Here we report cryo-EM structures of the HEAT-repeat protein Met18 from Saccharomyces cerevisiae, a key component of the CIA targeting complex (CTC) that identifies cytosolic and nuclear client proteins and delivers a mature iron-sulfur cluster. Met18 is a 118 kDa alpha solenoid protein comprised entirely of HEAT (Huntingtin, elongation factor 3 (EF3) repeats, protein phosphatase 1A, and the yeast kinase TOR1) repeats. ScMet18 has a curved S-shaped structure comprised of 23 HEAT-repeat (HR) units; each HR contains two α-helices that are connected by loops. We find that in the absence of other CTC proteins, Met18 adopts tetrameric and hexameric states.

To the best of our knowledge, our cryo-EM structure shows for the first time that ScMet18 can form an intertwined hexamer in the absence of other proteins. Our final model contains six copies of Met18 with each protomer consisting of residues 9-1029 with two loops missing at residues 225–241 and 315–337. The hexamer is 154 Å long and has both 3-fold and 2-fold symmetry. For all chains, the N-terminus is solvent-exposed, and the C-terminus is buried. Each chain of the hexamer interacts with 4 other chains (i.e., chain A touches chains B, C, D, and F, but not chain E). The hexamer is comprised of trimers and dimers where chains A, B, and C and chains D, E, and F can form trimers, and chains A and F, B and E, and C and D form dimers. Notably, the dimer from ScMet18 hexamer is not the same as the dimer observed in the crystal structure of MmMet18 in complex with DmCia2b-DmCia1. The curvature of ScMet18 differs from what has been observed previously with the MmMet18 protein in complex with DmCia2-DmCia1; there is a 44 Å shift in the N-terminus of ScMet18 compared to MmMet18. Notably, residues that appeared to be involved in binding Cia2 (R1010, R1013, R1020) are buried in both the hexameric and tetrameric states of ScMet18, indicating that ScCia2 cannot bind to ScMet18 without disrupting these higher order oligomeric states.

>MTPDELNSAVVTFMANLNIDDSKANETASTVTDSIVHRSIKLLEVVVALKDYFLSENEVERKKALTCLTTILAKTPKDHLSKNECSVIFQFYQSKLDDQALAKEVLEGFAALAPMKYVSINEIAQLLRLLLDNYQQGQHLASTRLWPFKILRKIFDRFFVNGSSTEQVKRINDLFIETFLHVANGEKDPRNLLLSFALNKSITSSLQNVENFKEDLFDVLFCYFPITFKPPKHDPYKISNQDLKTALRSAITATPLFAEDAYSNLLDKLTASSPVVKNDTLLTLLECVRKFGGSSILENWTLLWNALKFEIMQNSEGNENTLLNPYNKDQQSDDVGQYTNYDACLKIINLMALQLYNFDKVSFEKFFTHVLDELKPNFKYEKDLKQTCQILSAIGSGNVEIFNKVISSTFPLFLINTSEVAKLKLLIMNFSFFVDSYIDLFGRTSKESLGTPVPNNKMAEYKDEIIMILSMALTRSSKAEVTIRTLSVIQFTKMIKMKGFLTPEEVSLIIQYFTEEILTDNNKNIYYACLEGLKTISEIYEDLVFEISLKKLLDLLPDCFEEKIRVNDEENIHIETILKIILDFTTSRHILVKESITFLATKLNRVAKISKSREYCFLLISTIYSLFNNNNQNENVLNEEDALALKNAIEPKLFEIITQESAIVSDNYNLTLLSNVLFFTNLKIPQAAHQEELDRYNELFISEGKIRILDTPNVLAISYAKILSALNKNCQFPQKFTVLFGTVQLLKKHAPRMTETEKLGYLELLLVLSNKFVSEKDVIGLFDWKDLSVINLEVMVWLTKGLIMQNSLESSEIAKKFIDLLSNEEIGSLVSKLFEVFVMDISSLKKFKGISWNNNVKILYKQKFFGDIFQTLVSNYKNTVDMTIKCNYLTALSLVLKHTPSQSVGPFINDLFPLLLQALDMPDPEVRVSALETLKDTTDKHHTLITEHVSTIVPLLLSLSLPHKYNSVSVRLIALQLLEMITTVVPLNYCLSYQDDVLSALIPVLSDKKRIIRKQCVDTRQVYYELGQIPFE[6x]The mtr operon includes the genes to express three proteins: a decaheme cytochrome MtrA that inserts into the periplasmic side of a 28-strand transmembrane β-barrel MtrB9, and an outer membrane decaheme cytochrome MtrC that inserts into the extracellular side of MtrB. The outer membrane cytochromes MtrC, OmcA and MtrF are exported to the extracellular cell surface by the type II secretion system and S. oneidensis ΔomcA-ΔmtrC double mutants are severely compromised for respiratory mineral Fe(III) reduction and electron transfer to anodes in microbial fuel cells. Here we demonstrate a reversible transition of MtrC between cytochrome and flavocytochrome states that is controlled by the redox state of a conserved disulphide. All structures are formed of 4 domains, two multiheme domains that are flanked by two β-barrels with β-strands arranged in Greek key motifs.

To confirm the conformation of the CX8C motif we solved the x-ray crystal structure of S. oneidensis MR-1 MtrC. MtrC has substantial structural homology to MtrF, UndA and OmcA with two multi-heme domains flanked by two β-barrel domains and the same staggered deca-heme cross present in all structures. The structure reveals that, with approximate dimensions of 90 Å × 60 Å × 40 Å, MtrC is too large to fit into a 28-strand MtrB barrel and so would likely be mostly exposed on the surface of the cell. The ten hemes of MtrC are arranged in a ‘staggered-cross’ configuration that is a shared feature of the group of OMMC proteins. Alignment of the MtrC heme iron atoms with the iron atoms of UndA, MtrF and OmcA reveals that the heme arrangement of MtrC has a closer homology to MtrF with an r.m.s.d of 1.7 Å, than to UndA or OmcA with an r.m.s.d. of 2.1 Å. The conserved cysteines 444 and 453 of the CX8C motif form a single disulfide within domain III of MtrC. This disulfide is formed between a loop of 8 amino acids that contains a solvent exposed phenylalanine and valine. However, in domain III there is a hydrophobic cleft next to heme 7 that contains three phenylalanines, which in the UndA is occupied by an extra heme. The closest heme group to the MtrC disulfide is heme 7, suggesting that FMN would associate somewhere on domain III, in close proximity to heme 7. In the fumarate reductase of S. oneidensis MR-1 the edge-to-edge distance between the flavin cofactor and the nearest heme group is 7.5 Å, and this distance would place the MtrC flavin binding site approximately halfway between heme 7 and the disulfide bond.

> MKFKLNLITLALLANTGLAVAADGGGSDGNNGNDGSDGGEPAGSIQTLNLDITKVSYENGAPMVTVFATNEADMPVIGLANLEIKKALQLIPEGATGPGNSANWQGLGSSKSYVDNKNGSYTFKFDAFDSNKVFNAQLTQRFNVVSAAGKLADGTTVPVAEMVEDFDGQGNAPQYTKNIVSHEVCASCHVEGEKIYHQATEVETCISCHTQEFADGRGKPHVAFSHLIHNVHNANKAWGKDNKIPTVAQNIVQDNCQVCHVESDMLTEAKNWSRIPTMEVCSSCHVDIDFAAGKGHSQQLDNSNCIACHNSDWTAELHTAKTTATKNLINQYGIETTSTINTETKAATISVQVVDANGTAVDLKTILPKVQRLEIITNVGPNNATLGYSGKDSIFAIKNGALDPKATINDAGKLVYTTTKDLKLGQNGADSDTAFSFVGWSMCSSEGKFVDCADPAFDGVDVTKYTGMKADLAFATLSGKAPSTRHVDSVNMTACANCHTAEFEIHKGKQHAGFVMTEQLSHTQDANGKAIVGLDACVTCHTPDGTYSFANRGALELKLHKKHVEDAYGLIGGNCASCHSDFNLESFKKKGALNTAAAADKTGLYSTPITATCTTCHTVGSQYMVHTKETLESFGAVVDGTKDDATSAAQSETCFYCHTPTVADHTKVKMKGELKLEGKPIPNPLLGLDSTRTGHHHHHH>CGCGAAAAAACG[3x];>CGTTTTTTCGCG[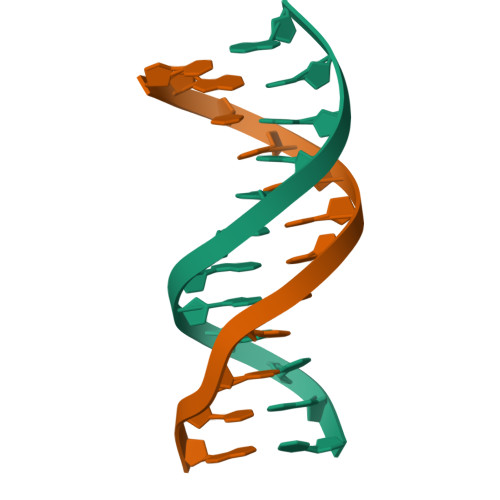3x]>[2x]GSHMNTSRFESLTGSVDVLFPEYDDPPSEPITLLKRWLATADVARVRE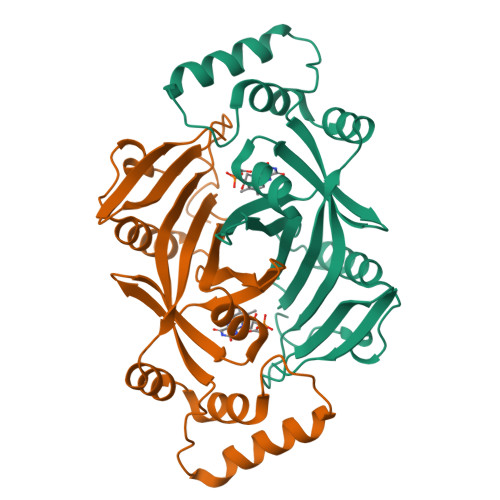PKALALATATSDGRISSRVIAFSSIDDRGVIFCTHSTSRKGRELTETGWASGLLYWRETGQQIMISGQAVPLEESENDKLWFGRSVPMHAMSSASHQSDELVDREALRAHAAELLALGVALPRPPRFVGYRLEPHEMEFWAASSDRLHRRLRYERDGNDWKTTQLQP CYCLOMETHYLTRYPTOPHAN | C12 H12 N2 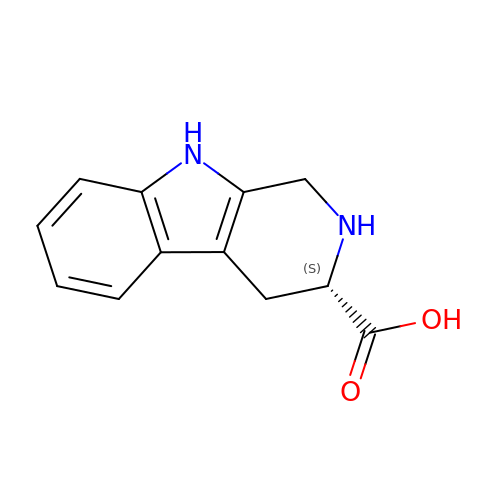O2 | FSNCEEGOMTYXKY-JTQLQIEISA-N>[16x]XGGLEEIAQGLEEIAKGLKKI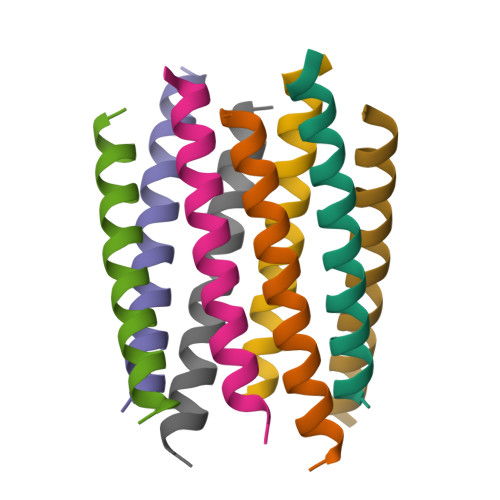AWGLKKIAQGGX>MGSSHHHHHHSSGLVPRGMTELLSREEYAAIAATLDLPQRAFIDGGFRDACGGRTFASTNPATGELLAQVAACDAEDVGHAVASARRAFEDGRWRSRTPAERKAALLRLAELLEEHLLELAVMESLDSGKPIRECQHTDLPETINTLRWHAELIDKIYDSTAPVGSAALAMVVREPIGVVGLVLPWNFPLLMLAWKIGPALAAGCSVVVKPAPETSLTALRVAELASQAGIPAGVFNVVPGGGREAGEPLGRHPDVAMVSFTGSTATGRLFLKYAAESNLKRVVLECGGKNPAVVMNDVEDLDLVAQHVVNGAFWNMGENCSASSRLIVHAEVREALLERIGAQLREWRMGDPLDPRNRLGALVSPAHFEKVRAYLDQARTERLAVRFGGATEAGIFVEPTVVDGVSPHSRLFREEIFGPLLSVTSFDDIDEAIALANDTVYGLAASAYTGSLRHALRLSREIRAGIVTVNCFGEGDASTPFGGYKESGFGGRDKSVWAHDQYT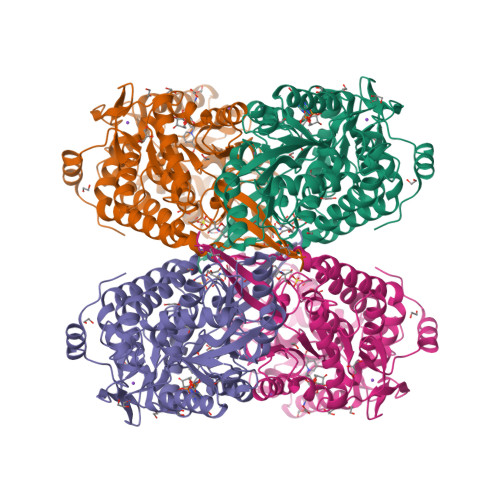ELKTIWIDAS[2x]>MASMTGGQQMGRGSEFMLQNNTDYPFEANNPYMYHENPMEEGLSMLKLANLAEAALAFEAVCQKEPEREEAWRSLGLTQAENEKDGLAIIALNHARMLDPKDIAVHAALAVSHTNEHNANAALASLRAWLLSQPQYEQLGSVNLQADVDIDDLNVQSEDFFFAAPNEYRECRTLLHAALEMNPNDAQLHASLGVLYNLSNNYDSAAANLRRAVELRPDDAQLWNKLGATLANGNRPQEALDAYNRALDINPGYVRVMYNMAVSYSNMSQYDLAAKQLVRAIYMQVGGTTPTGEASREATRSMWDFFRMLLNVMNRPDLVELTYAQNVEPFAKEFGLQSMLLEN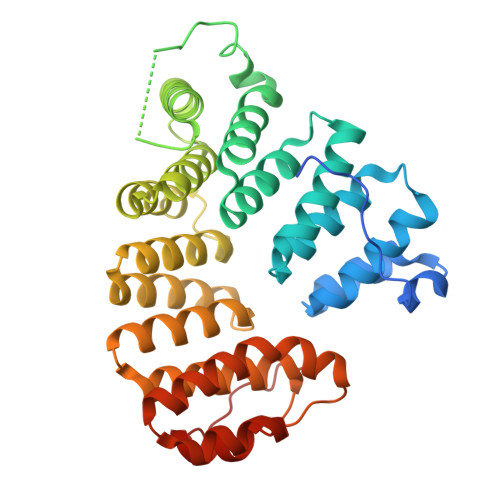LYFQ[2x]> MSAEKLFTPLKVGA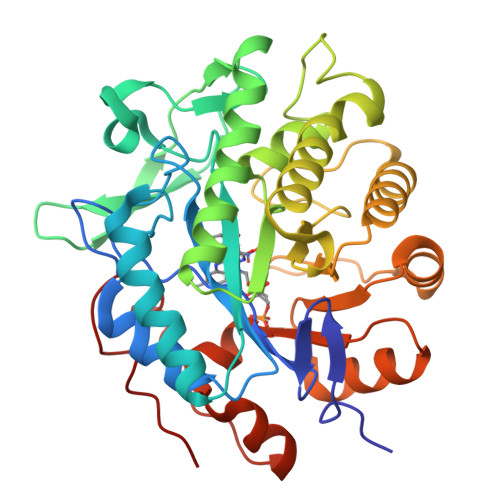VTAPNRVFMAPLTRLRSIEPGDIPTPLMGEYYRQRASAGLIISEATQISAQAKGYAGAPGLHSPEQIAAWKKITAGVHAEDGRIAVQLWHTGRISHSSIQPGGQAPVSASALNANTRTSLRDENGNAIRVDTTTPRALELDEIPGIVNDFRQAVANAREAGFDLVELHSAHGYLLHQFLSPSSNQRTDQYGGSVENRARLVLEVVDAVCNEWSADRIGIRVSPIGTFQNVDNGPNEEADALYLIEELAKRGIAYLHMSETDLAGGKPYSEAFRQKVRERFHGVIIGAGAYTAEKAEDLIGKGLIDAVAFGRDYIANPDLVARLQKKAELNPQRPESFYGGGAEGYTDYPSL>[4x]MWFGEFGGQYVPETLIEPLKELEKAYKRFKDDEEFNRQLNYYLKTWAGRPTPLYYAKRLTEKIGGAKIYLKRE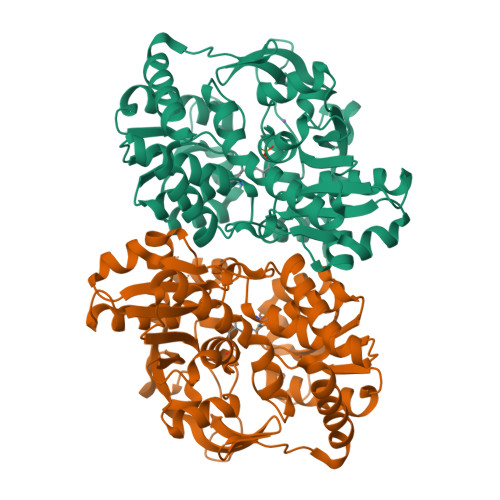DLVHGGAHKTNNAIGQALLAKFMGKTRLIAETGAGQHGVATAMAGALLGMKVDIYMGAEDVERQKMNVFRMKLLGANVIPVNSGSRTLKDAINEALRDWVATFEYTHYLIGSVVGPHPYPTIVRDFQSVIGREAKAQILEAEGQLPDVIVACVGGGSNAMGIFYPFVNDKKVKLVGVEAGGKGLESGKHSASLNAGQVGVFHGMLSYFLQDEEGQIKPTHSIAPGLDYPGVGPEHAYLKKIQRAEYVTVTDEEALKAFHELSRTEGIIPALESAHAVAYAMKLAKEMSRDEIIIVNLSGRGDKDLDIVLKVSGNV(~{E})-13-methyltetradec-2-enoic 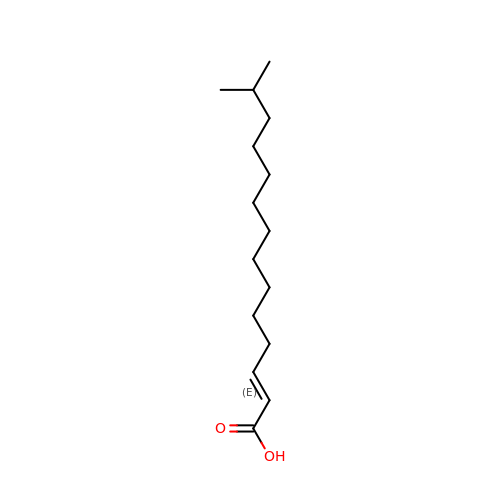acid | C15 H28 O2 | HNGBGNIRFVZXOQ-ACCUITESSA-N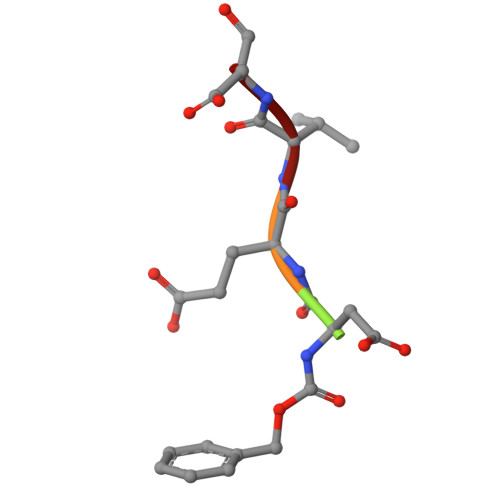> XDEVD>[2x]SNVLDGLKYAPSHEWVKHEGSVATIGITDHAQDHLGEVVFVELPEPGVSVTKGKGFGAVESVKATSDVNSPIS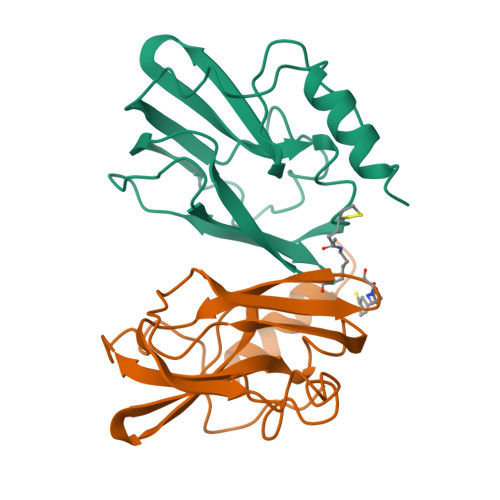GEVIEVNTGLTGKPGLINSSPYEDGWMIKIKPTSPDELESLLGAKEYTKFCEEEDAAH> ARTVVLITGCSSGIGLHLAVRLASDPSQSFKVYATLRDLKTQGRLWEAARALACPPGSLETLQLDVRDSKSVAAARERVTEGRVDVLVCNAGLGLLGPLEALGEDAVASVLDVNVVGTVRMLQAFLPDMKRRGSGRVLVTGSVGGLMGLPFNDVYCASKFALEGLCESLAVLLLPFGVHLSLIECGPVHTAFMEKVLG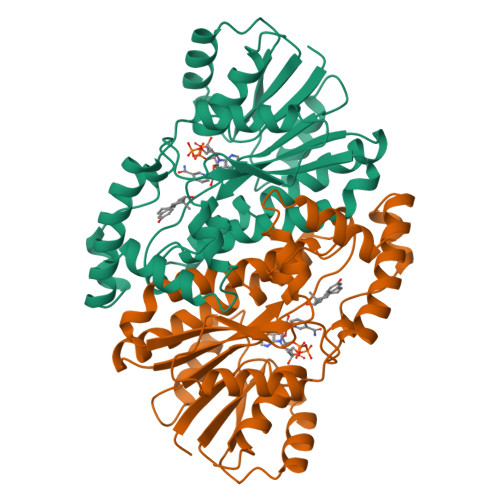SPEEVLDRTDIHTFHRFYQYLAHSKQVFREAAQNPEEVAEVFLTALRAPKPTLRYFTTERFLPLLRMRLDDPSGSNYVTAMHREVFGDVPA>MTKTKQAIHIDNIYWER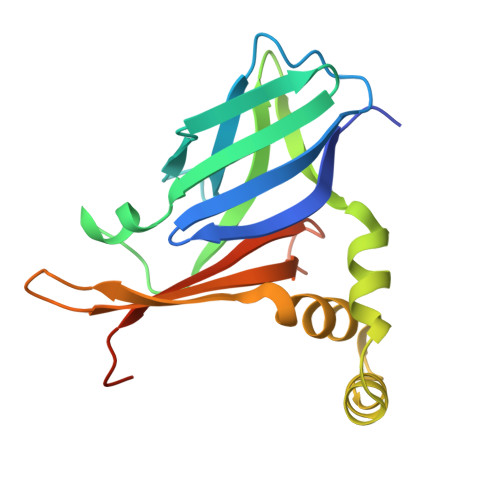VQLYIEGHSEGVDLTSGQFVLRNLTETKTLEANEMKIDGNTFICRFNVAILDDGYYLPMDKYLFVYHDQLEYIGQLNPNIIDQAYAALNEEQIEEYNELTTQNGKVNYLLAYDAKVFRKGGVSQHTVYTITPEIASDVNEFVFDIEITLPQEKSGGSLVPR[10x]> PISPIETVPVKLKPGMDGPKVKQWPLTEEKIKALVEICTEMEKEGKISKIGPENPYNTPVFAIKKKDSTKWRKLVDFRELNKRTQDFWEVQLGIPHPAGLKKKKSVTVLDVGDAYFSVPLDEDFRKYTAFTIPSINNETPGIRYQYNVLPQGWKGSPAIFQSSMTKILEPFKKQNPDIVIYQYMDDLYVGSDLEIGQHRTKIEELRQHLLRWGLTTPDKKHQKEPPFLWMGYELHPDKWTVQPIVLPEKDSWTVNDIQKLVGKLNWASQIYPGIKVRQLSKLLRGTKALTEVIPLTEEAELELAENREILKEPVHGVYYDPSKDLIAEIQKQGQGQWTYQIYQEPFKNLKTGKYARMRGAHTNDV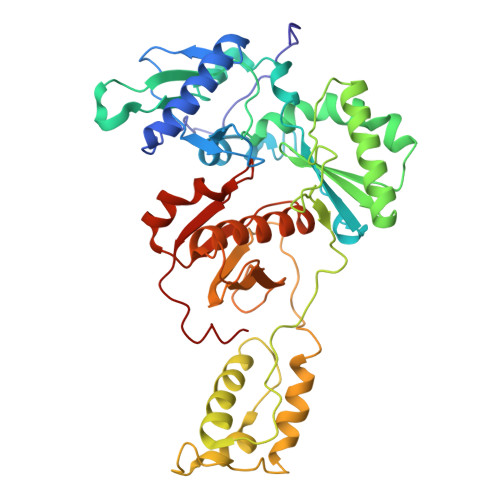KQLTEAVQKITTESIVIWGKTPKFKLPIQKETWETWWTEYWQATWIPEWEFVNTPPLVKLWYQLE>[4x]MQGFGVHAMMWSLNWDHESARRAIAGAADYGQDFIEIPLVDLPSVDTAHTRALLEKYGLRAACSLVLPEPAWASVRPEAAVAHLNAALDKAAEMGAEALTGVTYGGTSERTGFPPTQAEY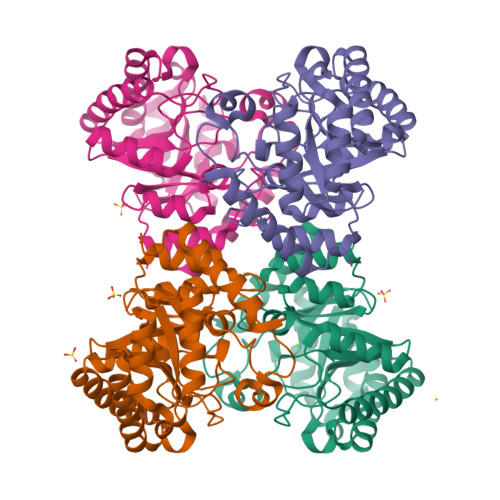DNLTRALSQSAGHAKTLGLQFGIEAVNRYENHLVNSAEQAVALVERIGADNIFVHLDTFHMNMEEKGIANGIIAAHDYLKYMHMSESDRGTPGFGNVAWDAVFAALAAIGFKGVLTLESFAAMPEEMAGAISTWRPVASGADEVLDKGLAFLRDKASQYRIFG> MDEFEMIKRNTSEIISEEELREVLKKDEKSAIIGFEPSGKIHLGHYLQIKKMIDLQNAGFDIIILLADLFAYLNQKGELDEIRKIGDYNKKVFEAMGLKAKYVYGSSFMLDKDYTLNVYRLALKTTLKRARRSMELIAREDENPKVAEVIYPIMQVNPLHYEGVDVAVGGMEQRKIHMLARELLPKKVVCIHNPVLTGLDGEGKMSSSKGNFIAVDDSPEEIRAKIKKAYCPAGVVEGNPIMEIA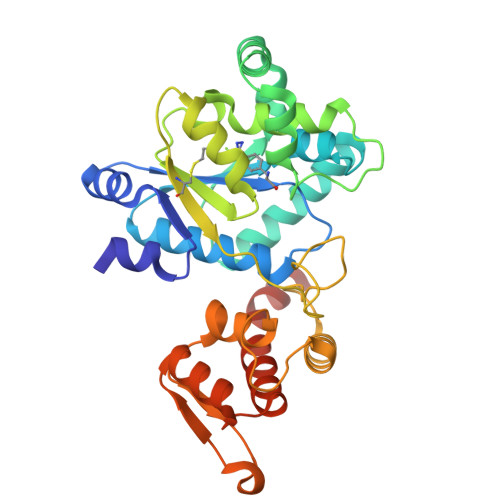KYFLEYPLTIKRPEKFGGDLTVNSYEELESLFKNKELHPMDLKNAVAEELIKILEPIRKRLLEHHHHHH>GPGFGGVFVGSFKIINYHLATIEERQSAIYVDWQSDVLVTPIAAHGRHQIARCKCNTGVYYCRHRDKSYPVCFEGPGIQWIEQNEYYPARYQTNVLLAAGPAEAGDCGGLLVCPHGVIGLLTA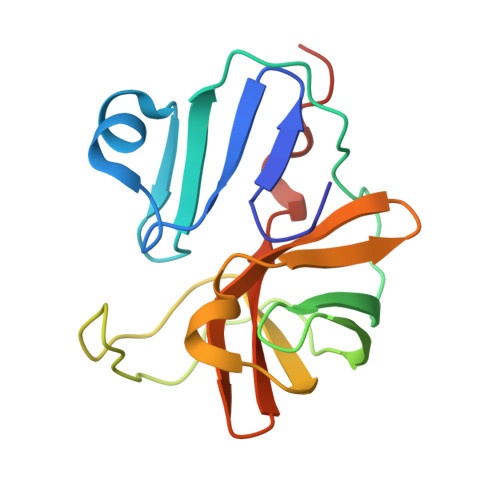GGGGIVAFTDIRNLLWLDTDAMEQ[6x]The netrin protein family is comprised of six members, the secreted netrins -1, -3, -4, -5 and the glycosylphosphatidylinositol (GPI)-anchored netrins-G1 and -G2 in mammals and exhibit homology to the N-terminal domains (LN-LEa1-3) of laminin short arms. Secreted netrins-1,-3 and -5 are homologous to the laminin γ1 chain, whereas netrin-4 (Net4) shares a higher identity to the β1 chain (50%). Our data demonstrate that Net4 not only strongly binds to laminin γ1 -thereby blocks efficiently laminin polymerization- but also actively disrupts pre-existing laminin networks in a non-enzymatic manner. Thus, our hypothesis is that Net4 is not a classic ligand activating a membrane receptor with a downstream signalling but rather a regulator of basal membrane maintenance, which indirectly impacts key functions such as axonal growth and angiogenesis.

In order to establish the structure-function relationship of Net4, we solved the crystal structure of Net4 lacking the C-terminal domain (Net4-ΔC) at 3.1 Å, revealing a head to stalk arrangement of 175 Å in length. The globular shaped N-terminal domain (LN) forms the head and the three and a half rod-like consecutive LE domains make up the stalk. The LN domain forms a β-sandwich jelly-roll motif with a front face composed of sheet S5-S2-S7 and a dorsal face composed of sheet S4-S3-S6-S1. The topology of this domain is similar to the N-terminal domain of Net1; however, the closest structural homologue is the short arm of laminin β1. The LN domain is stabilized by a complex pattern of disulfide bridges composed of 12 cysteine residues. Two disulfide bridges between cysteine residues 72–236 and 191–234, absent in any current netrin or laminin structure, hold the S6-S7 loop in place. Furthermore, there is clear electron density for glycan additions at three asparagine-linked glycosylation sites, Asn56, Asn163, and Asn353. Remarkably, Net4 is the first member of the netrin family with no N-linked glycan attachment at the dorsal face of the N-terminal domain. Net4-ΔC has a total accessible surface area of ∼28,000 Å2 and reveals extensive inter-domain contacts between the LN domain and subdomain LE1. Structural analysis of Net4 and previously published Net1 complex structures reveals incompatibility between the binding residues of Net1 and equivalently positioned residues of Net4.

> CEKACNPRMGNLALGRKLRADTMCGQNATELFCFYSENADLTCRQPKCDKCNAAHSHLAHPPSAMADSSFRFPRTWWQSAEDVHREKIQLDLEAEFYFTHLIMVFKSPRPAAMVLDRSQDFGKTWKPYKYFATNCSATFGLEDDVVKKGAICTSRYSNPFPCTGGEVIFRALSPPYDIENPYSAKVQEQLKITNLRVRLLKRQSCPCQINDLNAKPHHFMHYAVYDFIVKGSCFCNGHADQCLPVEGFRPIKAPGAFHVVHGRCMCKHNTAGSHCQHCAPLYNDRPWEAADGRTGAPNECRTCKCNGHADTCHFDVNVWEASGNRSGGVCNNCQHNTEGQHCQRCKPGFYRDLRRPFSAPDACKACSCHPVGSAILPFSSVTFCDPSNGDCPCKPGVAGPHCDRCMVGYWGFGDYGCRPCDCAGSCDPLTGDC> MKIIAYGARVDEIQYFKQWAKDTGNTLEYHTEFLDENTVEWAKGFDGINSLQTTPYAAGVFEKMHAYGIKFLTIRNVGTDNIDMTAMKQYGIRLSNVPAYSPAAIAEFALTDTLYLLRNMGKVQAQLQAGDYEKAGTFIGKELGQQTVGVMGTGHIGQVAIKLFKGFGAKVIAYDPYPMKGDHPDFDYVSLEDLFKQSDVIDLHVPGIEQNTHIINEAAFNLMKPGAIVINTARPNLIDTQAMLSNLKSGKLAGVGIDTYEYETEDLLNLAKHGSFKDPLWDELL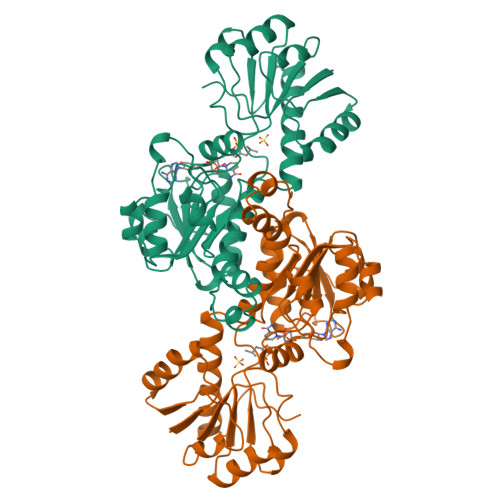GMPNVVLSPHIAYYTETAVHNMVYFSLQHLVDFLTKGETSTEVTGPAK> MISLNGYGRFGLQYVEDRGVGLEDTIISSRLRINIVGTTETDQGVTFGAALAM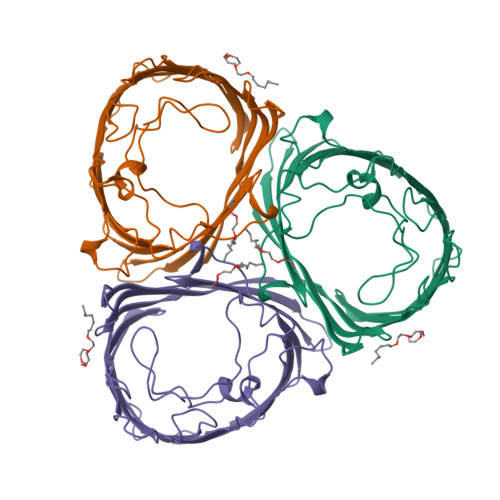QWDDGDAFAGTAGNAAQFWTSYNGVTVSVGNVDTAFDSVALTYDSEMGYEASSFGDAQSSFFAYNSKYDASGALDNYNGIAVTYSISGVNLYLSYVDPDQTVDSSLVTEEFGIAADWSNDMISLAAAYTTDAGGIVDNDIAFVGAAYKFNDAGTVGLNWYDNGLSTAGDQVTLYGNYAFGATTVRAYVSDIDRAGADTAYGIGADYQFAEGVKVSGSVQSGFANETVADVGVRFDF tridecylboronic acid | C13 H29 B O2 | 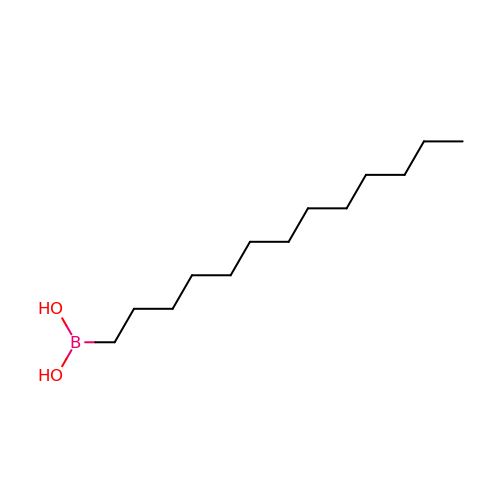IBKXABQGVIIFFS-UHFFFAOYSA-N>[2x]MMYRAPKTEKGKESLNKILDASVELIADKGFLSTSINDITSKAGVAYGLFYFYFKSKHDILDEIIRQFNRNMRYYLKTYTQNLDSRIDVEKVGMKKFLEWMNENKKYYKIFIETQVHRPDIYKWHFMKLAERYTTGLSEAMRRGEIINVDPELLSYVLIGIAHMLGKRYVLWSNSGLTLKQQRDLDLIIENMLTPR

FadRSa, of which we show that it displays structural similarities with bacterial TetR-like FadR regulators, is an archaeal member of the widespread prokaryotic TetR family. Each subunit displays two functional domains: an N-terminal helix-turn-helix (HTH) DNA-binding domain (α1–α3) and a C-terminal domain (α4–α9) of which α8 and α9 stabilize dimerization. The finding that FadRSa represses the Saci_1103-Saci_1126 gene cluster and that it is responsive to acyl-CoA molecules acting as inducers in vitro strongly suggests that intracellularly present acyl-CoA molecules cause a derepression and thus higher transcriptional expression of the gene cluster in vivo.

Next, we prepared FadRSa crystals in the presence of lauroyl–CoA (C12:0-CoA) and solved the FadRSa–lauroyl–CoA cocrystal structure to a resolution of 1.90 Å. In contrast to the initial structure showing an acyl-CoA derivative bound to only one of the subunits, in this structure, both subunits of the dimer harbor a lauroyl–CoA molecule. The orientation of the ligand-binding pockets within the protein and the binding mode of the ligand is completely different in FadRSa as compared to the characterized bacterial FadR proteins. In contrast to the ligand entering the pocket from within the dimer interface as in bacterial FadR regulators, in the FadRSa structure the ligand enters the protein from the outer surface of the protein completely opposite to the dimer interface. Further, for each ligand-binding pocket only a single FadRSa subunit is involved in ligand interaction in contrast to two subunits in the bacterial FadR regulators. The lauroyl chain is deeply buried into a tunnel-like binding pocket formed in between helices α4–α7 and is entirely surrounded by hydrophobic residues such as Phe68, Phe97, Phe111, and Phe126. Alanine substitution of the CoA-interacting residues Arg73 and Arg86 confirmed their importance for the ligand response. Subtle differences were noted in the relative orientation of the HTH motifs within a dimer with the binding of lauroyl–CoA causing the distance between the two α3 helices to be enlarged from an average 37.0–43.2 Å (measured as the Cα–Cα distance of Tyr51 residues located in α3). As a consequence, the increased distance between the α3 helices makes the dimeric FadRSa conformation suboptimal for interaction in consecutive major groove segments. Besides the α3 helix, the α2 helix is shifted by an average distance of 7.9 Å and the α4 helix is displaced with an angle of 9°.> GPEPDMISVFIGTWNMGSVPPPKNVTSWFTSKGLGKTLDEVTVTIPHDIYVFGTQENSVGDREWLDLLRGGLKELTDLDYRPIAMQSLWNIKVAVLVKPEHENRISHVSTSSVKTGIANTLGNKGAVGVSFMFNGTSFGFVNCHLTSGNEKTARRNQNYLDILRLLSLGDRQLNADDISDRFTHLFWFGDLNYRLDMDIQEILNYISRKEFEPLLRVDQLNLEREKHKVFLRFSEEEISFPPTYRYERGSRDTYAWHKQKPTGVRTNVPSWCDRILWK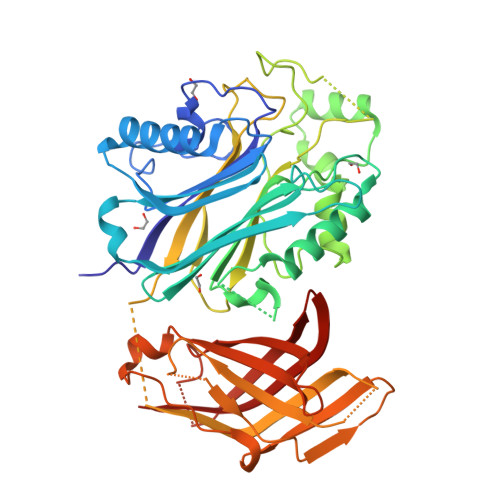SYPETHIICNSYGCTDDIVTSDHSPVFGTFEVGVTSQFISKKGLSKTSDQAYIEFESIEAIVKTASRTKFFIEFYSTCLEEYKKSFENDAQSSDNINFLKVQWSSRQLPTLKPILADIEYLQDQHLLLTVKSMDGYESYGECVVALKSMIGSTAQQFLTFLSHRGEETGNIRGSMKVRVPTER>ADATDDYPIPNRIMRTPCTAEQIMAAARDVEPVYYERYMTDYKNKPPHVQQAARDRIHWFFSMDYAGRRQYSENTATDAFFEQLAWMWPNWAKLFFNNKGVAANTTDVCEQYPPDDMSVWNWDDDDK[2x]

To acquire iron from the host, M. tuberculosis uses the siderophores called mycobactins and carboxymycobactins. In this study, we show that the mycobacterial core protein Rv0455c, a 14-kDa exported protein of previously unknown function, is required for siderophore secretion by M. tuberculosis. Similar quantities of Rv0455c protein are localized in the periplasm of M. tuberculosis and are secreted into the culture medium, but Rv0455c exerts its function in siderophore secretion in the periplasm. Rv0455c homologs are highly conserved in mycobacteria (>65% similarity) and are encoded by genes classified as mycobacterial core genes.

To circumvent these difficulties, we examined the close homolog MSMEG_3494 of M. smegmatis, which shares 66% similar amino acids with Rv0455c and has the same function. The three-dimensional structure of MSMEG_349433–153 was solved by X-ray crystallography and refined to 2.1 Å. To this end, the crystal was soaked with sodium bromide, and the phases were determined by multiwave anomalous dispersion (MAD) using the bromide ions as the source of anomalous scattering. The unit cell contained two molecules of MSMEG_349433–153 and 11 bromide ions with ~42% of the volume being occupied by solvent molecules. MSMEG_349433–153 adopts a novel structure consisting of a helical bundle with four single turn α-helices and five longer α-helices. A disulfide bond between C49 and C140 connects the N-terminus of helix 2 and the C-terminus of helix 8, establishing a cinch-like topology. These two cysteines are conserved across all members of the DUF5078 homology, indicating that the disulfide bond plays an important role in structure stabilization. In addition, we found that other evolutionarily conserved amino acids clustered predominantly in two distinct surface-exposed patches: the interface between the flexible N-terminus and helix 5 (patch 1), and the interfacial region of helices 2, 3, 7, and 8, (patch 2). Analysis of the electrostatic potential map of MSMEG_349433–153 revealed a highly electropositive surface for patch 2, which may form an interaction interface accommodating proteins or molecules with negatively charged domains or moieties. However, the lack of chemical shift perturbations by NMR spectroscopy indicated that the close Rv0455c homolog MSMEG_3494 does not interact with carboxymycobactin. This finding is consistent with the absence of a deep cleft in the crystal structure of MSMEG_3494 and in the identical structure of Rv0455c predicted by AlphaFold36.> ASMNPFMNTNPFLEELDQPIPSNAAKPISEETRDLFLSDGQTIPSSQEKIATIHEYLLEHKELEEAMFSLISQGRGRSLINMVVKSALNIETQSREVTGERRQRLERKLRNLENQGIYVDESKIMSRGRISKEDTELAMRIARKNQKDAKLRRIYSNNASIQESYTVDDFVSYWMEQESLPTGIQIAMWLKGDDWSQPIPPRVQRRHYDSYIMMLGPSPTQEQADAVKDLVDDIYDRNQGKGPSQEQ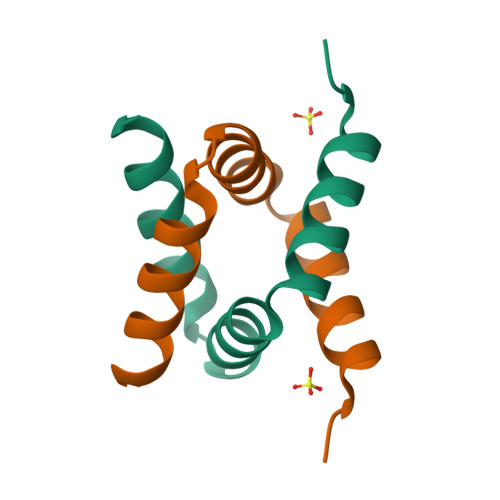ARELSHAVRRLISHSLVNQPATAPRVPPRRIVSAQTAQTDPPGRRAALDRLRRVRGEDNDIV4-[(2R)-2-(AMINOMETHYL)-2-(HYDROXYMETHYL)-5-OXOPYRROLIDIN-1-YL]-3-[(1-ETHYLPROPYL)AMINO]BENZOIC ACID | C18 H27 N3 O4 | 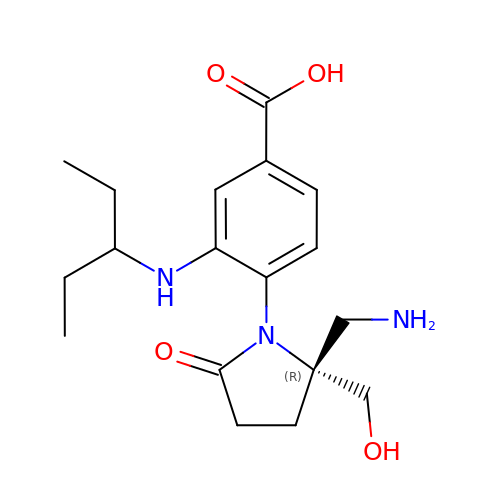ZEZFFRWWHKSMEB-GOSISDBHSA-N> SAPANAVAADNATAIALKYNQDATKSERVAAARPG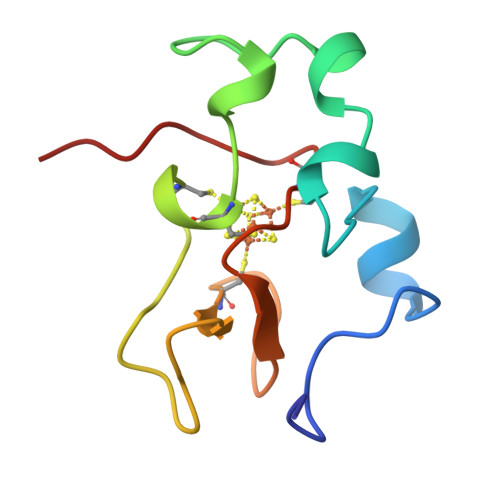LPPEEQQCANCQFMQADAAGATDEWKGCQLFPGKLINVNGWCASWTLKAG>KNEPVLDIDGEELRAGEQYYVVSAIWGPGGGGLALGRLTDQKCPEIVVQRRSDSDYGTPVIFHNLDTKDDIVRLSTDFNVEFVPIRDRLCLTSTVWKIDDYDTSTGKWWVTTDGVKGNPGPHTLQSWFKIEKSGNFGYKFNFCPSVCESCITLCGDIGRYGHDGQIRLALAESGWP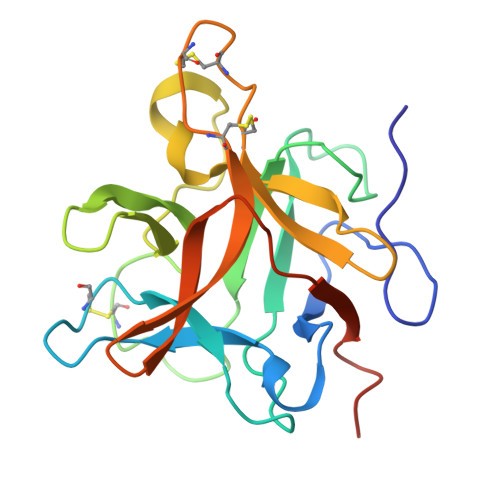FVFQKASSTIKQVVNAKN[2x]> TEDMEDAWQDDEYFGNYGTLRLHLEMLSDKPRTETYRQVILSNSAALREKVVLDLGCGTGVISLFCALLAKPAGVYAVEASSMAEHTEELVKQNGCDGVVTVFQERAENLTLPTKVDVLVSEWMGNCLLFEYMLESVLLARDRWLKKGGMMWPSSACLTIVPCQA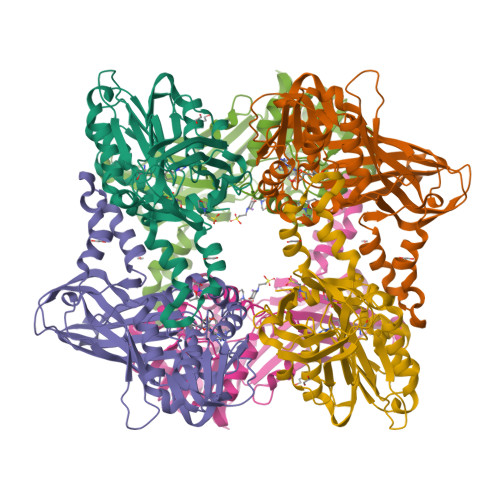FSDYRQKVEFWENPYGLNFSYLQSLAQKEFLSKPKFSHHLQPEDCLSTPADVITLDMVTIQVSDLERLKGEFTFTVEKSGMFHGFTVWFSAHFQCLEEDGPSIELNTGPYSEITHWKQTLFMLDAPVSVEEGDIIAGSIRLQRNPIWRRHLSITFLWNINSTEVSTVKTKCFPMWR> LAAVSVDCSEYPKPACPKDYRPVCGSDNKTYSNKCNFCNAVVE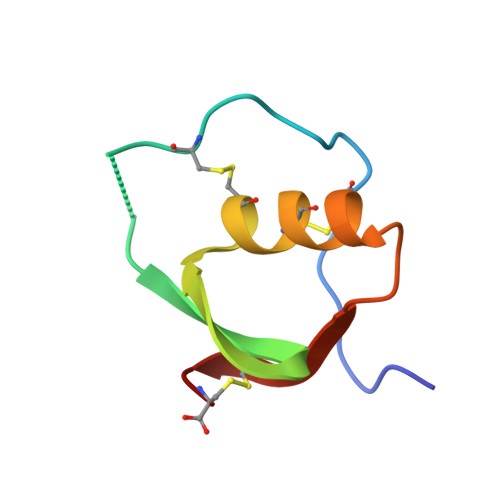SNGTLTLNHFGKC>[6x]MSHHHHHHGSSGSILNDYKRKTEGSVFWAQRARSVMPDGVTADTRVFDPHGLFISDAQGVHKTDVDGNVYLDFFGGHGALVLGHGHPRVNAAIAEALSHGVQYAASHPLEVRWAERIVAAFPSIRKLRFTGSGTETTLLALRVARAFTGRRMILRIATHYHGWHDFSASGYNSHFDGQPAPGVLPEI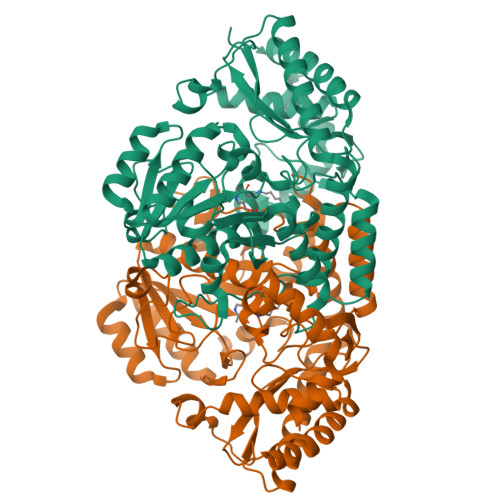AKNTLLIRPDDIEGMREVFAQHGSDIAAFIAEPVGSHFGVTPVSDSFLREGAELARQYGALFILDEVISGFRVGNHGMQALLDVQPDLTCLAKASAGGLPGGILGGREDVMGVLSRGSDRKVLHQGTFTGNPITAAAAIAAIDTILEDDVCAKINDLGQFAREAMNHLFARKGLNWLAYGRFSGFHLMPGLPPNTTDTGSITRAEVARPDVKMIAAMRMALILEGVDIGGRGSVFLSAQHEREHVEHLVTTFDRVLDRLADENLLSWQPTNLSGNQS>[6x]GGGMFNYTVLPSTSLAVGYYYNFLREI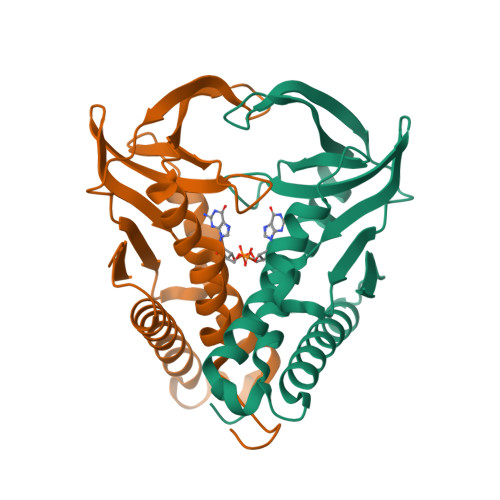LEAFNNQKSIQIILERDRTGKPTKTIDYEIKKPYPTIEIRVPQNLASLKKEVLTWNTSEYKQIFINAASRTYPFFLQGEFKEDQILSIFDIPTTLYASYLTIKELFTDSFLKTQNNERKLINKEIRNFERTLSKLIDDTIEEKFYKFTIY[1-PENTADECANOYL-2-DECANOYL-GLYCEROL-3-YL]PHOSPHONYL 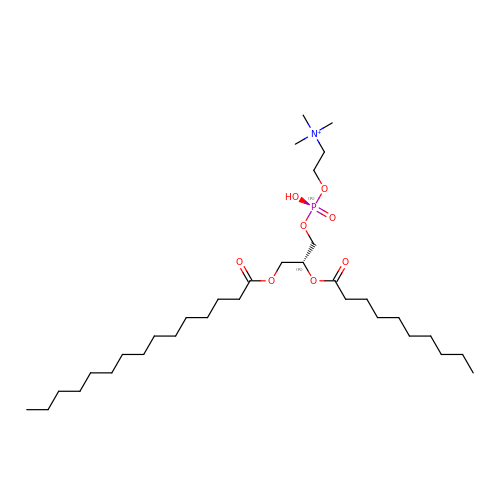CHOLINE | C33 H67 N O8 P | YAOVLDDMIGILIT-WJOKGBTCSA-O>MEIMEFEEAFKEVYEMVKPKYKLFTAGPVACFPEVLEIMKVQMFSHRSKEYRKVHMDTVERLREFLEVEKGEVLLVPSSGTGIMEASIRNGVSKGGKVLVTIIGAFGKRYKEVVESNGRKAVVLEYEPGKAVKPEDLDDALRKNPDVEAVTITYNETSTGVLNPLPELAKVAKEHDKLVFVDAVSAMGGADIKFDKWGLDVVFSSSQKAFGVPPGLAIGAFSERFLEIAEKMPERGWYFDIPLYVKYLKEKESTPSTPPMPQVFGINVALRIIEKMGGKEKWLEMYEKRAKMVREGVREIGLDILAEPGHESPTITAVLTPPGIKGDEVYEAMRKRGFELAKGYGSVKEKTFRIGHMGYMKFEDIQEMLDNLREVINELKKQK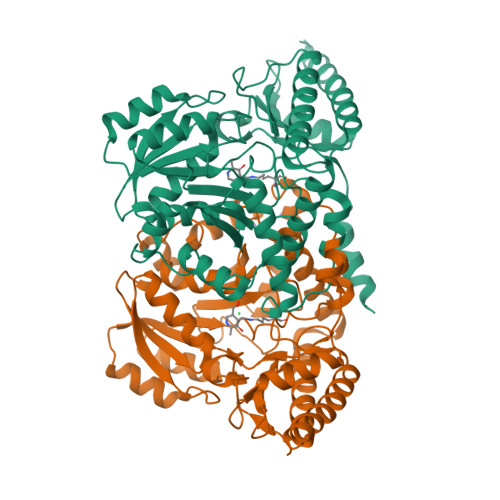GIN[2x]> SNIQTGAERMPHDLSHLGFLAGQIGRLITISTTPVIAGDS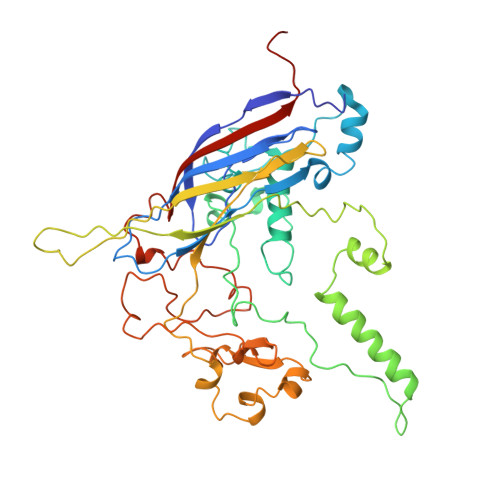FEMDAVGALRLSPLRRGLAIDSTVDIFTFYVPHRHVYGEQWIKFMKDGVNATPLPTVNTTGYIDHAAFLGTINPDTNKIPKHLFQGYLNIYNNYFKAPWMPDRTEANPNELNQDDARYGFRCCHLKNIWTAPLPPETELSRQMTTSTTSIDIMGLQAAYANLHTDQERDYFMQRYRDVISSFGGKTSYDADNRPLLVMRSNLWASGYDVDGTDQTSLGQFSGRVQQTYKHSVPRFFVPEHGTMFTLALVRFPPTATKEIQYLNAKGALTYTDIAGDPVLYGNLPPREISMKDVFRSGDSSKKFKIAEGQWYRYAPSYVSPAYHLLEGFPFIQEPPSGDLQERVLIRHHDYDQCFQSVQLLQWNSQVKFNVTVYRNLPTTRDSIMTS>[4x]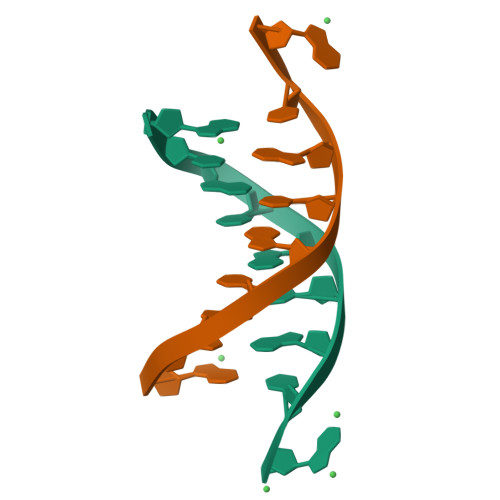CGTATATACG The 12-kDa FK506-binding protein (FKBP12) is a ubiquitously expressed peptidyl-prolyl isomerase with considerable homology between fungal pathogens and is thus a prime candidate for future targeting efforts to generate a panfungal strategy. PPIase proteins all catalyze the cis/trans isomerization of peptide bonds N terminal to proline residues in polypeptide chains. In addition to its role as a PPIase, FKBP12 is a member of the immunophilin family and is the target of the immunosuppressive drugs FK506 and rapamycin. Three extended loops, which have been called the 40s loop (between β2 and β3), the 50s loop (between β3′ and α1), and the 80s loop (between β4 and β5), surround a deep active-site pocket that binds both FK506 and rapamycin.

Another clinically important and often antifungal-resistant Candida species, C. glabrata, contains a glycine at this location, suggesting that this protein would not form the intermolecular interaction. To test this prediction, we determined the structures of C. glabrata FKBP12 in its apo and FK506-bound states. Examination of the packing revealed a close contact between the 80s loop of one subunit and an adjacent molecule in the apo crystals. However, here the 80s loop is not inserted into the active site of the neighboring molecule. Hence, as predicted, the C. glabrata FKBP12 structure shows no evidence of an intermolecular self-catalysis-like binding event. Strikingly, the C. albicans and A. fumigatus FKBP12 apo structures all revealed the deep insertion of a proline located in the 80s loop into the ligand-binding pocket of a neighboring FKBP12 subunit. This interaction was not observed in the C. glabrata structure, which does not have the corresponding proline residue.

> AMSETIEGGVKIDRLSPGDGKTFPKQGDLVTIHYTGTLENGQKFDSSVDRGSPFQCNIGVGQVIKGWDAGIPKLSVGEKARLTIPGPYAYGPRGFPGLIPPNATLIFDVELLKVN> MTTLTLSEAAPLLKKEFREGRLIPFLGAGFSKPLKLPDGSQLIASLAKTLGFEPELFDMHGRFEQLAEFFAISAPNRLQRLVYEMSLSFDSAEA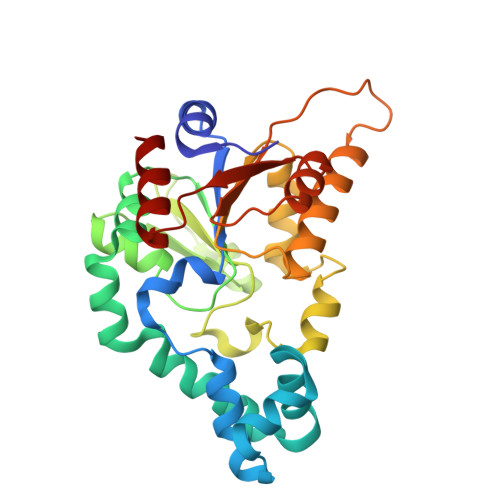EALREKSPMHRALAALDWRTIYTTNYDKHVEGALRDAGKQAAVLASFADFQGPRARDVCEVIKFHGTLDQPDTIVLTESSYFQRMALDAPPDQRLRADLLANSFLFIGYSFSDTNIRYIWYRMNQLREQSQLGVKHSQARRCFFATHGAGLVQPDILQQWNIDVIQLDPTDKSASVARLLESIA>[4x]MSTEKFTITEHLVPGSHIREYPGSTVNQEDVLKIHVKQYTPKREGPVPDDAITFIATHGVGLPKELYEPLWDELLDQASGFHIRAIWMADVASMNQSGIHNEDKLSMDCSW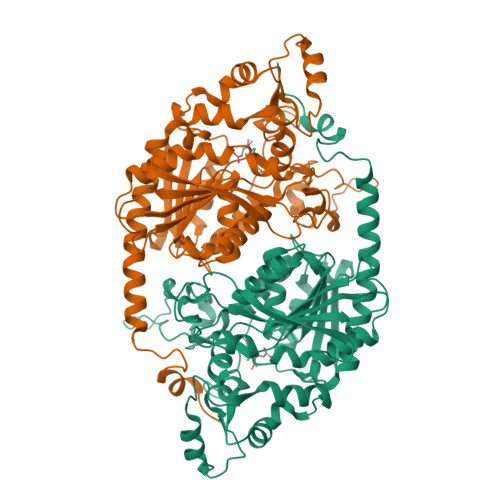MDHARDLLLMINHFRDQMPRPLVGIGHAFGGNIITNLAYLHPRLFTTLLLLDPLIQLSPPSLGFGTDAPSAINYTLWRDDVWPSREVAIRANRAIMQGMDPRCLDRMTKHFFRDLPTPLYPDVEAIKALFGTTADSTTTPVTLTTPKYHELVAQIRQNFNARDPKTGRIEVPRDTHADMDPLVAYIPLYRPEPRSTFRRLETLRPSCLWVIAGATFLNIDEIREGVKICGSGIGGSGGVPDGRVREVVLPGFGHLMPFQEVKTVAETCIVWLQQEMDRFRQTERQWKEDRDGKSHLAVEENWYKVLKPIPSGRKKRNDKGKL> SMEMPV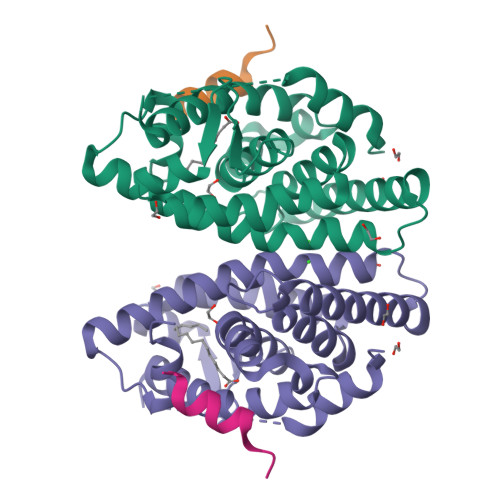DRILEAELAVEQKSDQGVEGPGGTGGSGSSPNDPVTNICQAADKQLFTLVEWAKRIPHFSSLPLDDQVILLRAGWNELLIASFSHRSIDVRDGILLATGLHVHRNSAHSAGVGAIFDRVLTELVSKMRDMRMDKTELGCLRAIILFNPDAKGLSNPSEVEVLREKVYASLETYCKQKYPEQQGRFAKLLLRLPALRSIGLKCLEHLFFFKLIGDTPIDTFLMEMLEAPHQLA;> KHKILHRLLQDSSY> AKYVCKICGYIYDEDAGDPDNGV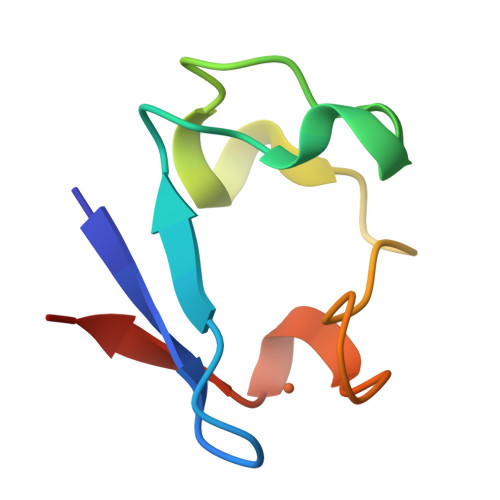SPGTKFEEIPDDWVCPICGAPKSEFEKLED> MWTLSRPCLAAVRTAVLCQKKQTAAGYMASAGKVGNEEKWAQAAMEYIHEKNHVNDARKRQQDVDQER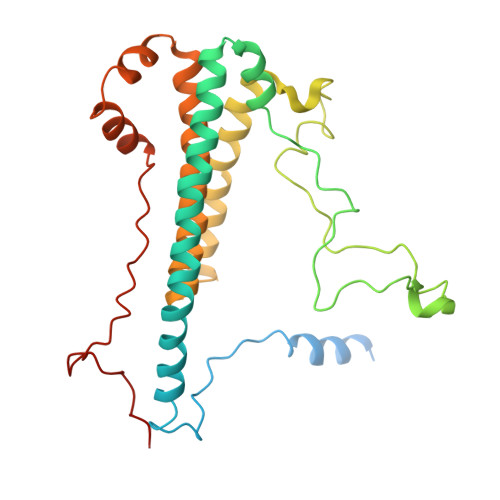SIANAYDRYSAVSEAKFDERLSRLIARMSEALEEMRNLGLEEALEEAVLLNSEQPPGHYRRPSLTPPLAGYEPGFGLDVPQLRSQQAEYPPLRRPTDWLEFGEGGADDFPYVDTHKIEDLTAKHEAQLEEQHGVLREAAPLTGVEGEGWEAYVALHRKALARQHLIMDLHNDPELRDKYNADEAFRAAEWERRGMGALSIEAPLERDLELHYAQVPAYEAFRSH> ARKS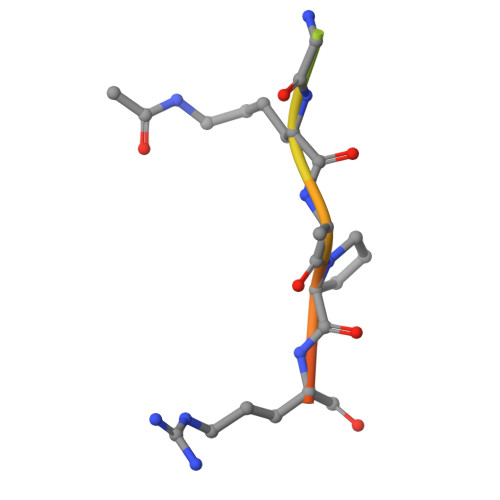TGGKAPRKQL>GAHMFKIPGFGKAAANHTPPDMTNMDTRTRHLKVSNCPNNSYALANVAAVSPNDFPNNIYIIIDNLFVFTTRHSNDIPPGTIGFNGNQRTWGGWSLNQDVQAKAFDLFKYSGKQSYLGSIDIDISFRARGKAVSTVFDQDELAKQFVRCYESQIFSPTQYLIMEFQGHFFDLKIRNVQAIDLGDIEPTSAVATGIETKGILTKQTQINFFKGRDGLVNLKSSNSLRPRSNAVIRPDFKFEDLGVGGLDKEFTKIFRRAFASRIFPPSVIEKLGISHVKGLLLYGPPGTGKTLIARKIGTMLNAKEPKIVNGPEILSKYVGSSEENIRNLFKDAEAEYRAKGEESSLHIIIFDELDSVFKQRGSRGDGTGVGDNVVNQLLAKMDGVDQLNNILVIGMTNRKDLIDSALLRPGRFEVQVEIHLPDEKGRLQIFDIQTKKMRENNMMSDDVNLAELAALTKNFSGAEIEGLVKSASSFAINKTVNIGKGATKLNTKDIAKLKVTREDFLNALNDVTPAFGISEEDLKTCVEGGMMLYSERVNSILKNGARYVRQVRESDKSRLVSLLIHGPAGSGKTALAAEIALKSGFPFIRLISPNELSGMSESAKIAYIDNTFRDAYKSPLNILVIDSLETLVDWVPIGPRFSNNILQMLKVALKRKPPQDRRLLIMTTTSAYSVLQQMDILSCFDNEIAVPNMTNLDELNNVMIESNFLDDAGRVKVINELSRSCPNFNVGIKKTLTNIETARHDEDPVNELVELMTQSA[6x];>GMSDPVELLKRAEKKGVPSSGFMKLFSGSDSYKFEEAADLCVQAATIYRLRKELNLAGDSFLKAADYQKKAGNEDEAGNTYVEAYKCFKSGGNSVNAVDSLENAIQIFTHRGQFRRGANFKFELGEILENDLHDYAKAIDCYELAGEWYAQDQSVALSNKCFIKCADLKALDGQYIEASDIYSKLIKSSMGNRLSQWSLKDYFLKKGLCQLAATDAVAAARTLQEGQSEDPNFADSRESNFLKSLIDAVNEGDSEQLSEHCKEFDNFMRLDKWKITILNKIKESIQQQEDDLL[3x];> GASHMSSSTPFDPYALSEHDEERPQNVQSKSRTAELQAEIDDTVGIMRDNINKVAERGERLTSIEDKADNLAVSAQGFKRGANRVRKAMWYKDLKMK;> GASHMSYNNPYQLETPFEESYELDEGSSAIGAEGHDFVGFMNKISQINRDLDKYDHTINQVDSLHKRLLTEVNEEQASHLRHSLDNFVAQATDLQFKLKNEIKSAQRDGIHDTNKQAQAENSRQRFLKLIQDYRIVDSNYKEENKEQAKRQYMIIQPEATEDEVEAAISDVGGQQIFSQALLNANRRGEAKTALAEVQARHQELLKLEKSMAELTQLFNDMEELVIEQQENVDVIDKNVEDAQLDVEQGVGHTDKAVKSARKARKNKIR;> GASHIKFTKQSSVASTRNTLKMAQDAERAGMNTLGMLGHQSEQLNNVEGNLDLMKVQNKVADEKVAELKKLNRSILAVHVSNPFNSKRRRREREEQLKNRKIEEKLMREQTSQQLSQSTQRIEGAMNANNNISEVRERYQRKNVLEKAKRYQFENDEEDDEMELEIDRNLDQIQQVSNRLKKMALTTGKELDSQQKRLNNIEESTDDLDINLHMNTNRLAGI

SNARE (soluble N-ethylmaleimide-sensitive factor (NSF) attachment protein receptor) proteins drive membrane fusion at different cell compartments as their core domains zipper into a parallel four-helix bundle. After fusion, these bundles are disassembled by the AAA+ (ATPase associated with diverse cellular activities) protein Sec18/NSF and its adaptor Sec17/α-SNAP to make them available for subsequent rounds of membrane fusion. The disassembly requires multiple ATP hydrolysis events in the presence of Mg2+; as few as six ATP hydrolysis events are sufficient. The side-loading and side-release mechanism explains how Sec18/NSF can disassemble SNAREs with constrained topologies.

We chose the Sso1–Sec9–Snc1/Snc2 complex (referred to as the ySNARE complex) because each component of this complex crosslinked with high confidence to the D2 domain of Sec18 (Snc1 is highly homologous to Snc2). We prepared the y20S complex in a nonhydrolyzing condition and, after single-particle cryo-EM data collection and processing, we obtained 381,591 high-quality particles that yielded eight three-dimensional (3D) classes into which models were built. In the structures of all eight classes, Sso1 is threaded through the D1 pore of Sec18. A characteristic phenylalanine side-chain density in Sso1 is present at the same position relative to Sec18 in all classes, allowing for reliable indexing of Sso1. The nucleotide states and the arrangements of D1 around the substrate were also the same among all eight classes, with the ADP-engaged E protomer forming the top of a spiral staircase of tyrosine residues. Protomers D, B and C were all ATP bound and formed the middle of the staircase. The bottom protomer, A, formed the base of the staircase. Protomer F, with no apparent density for nucleotide in D1, was not associated with Sso1. Given that this charge distribution is replicated between each pair of D2 subdomains around the D2 surface, it is unsurprising that the Habc domain adopts multiple corresponding rotational states over the eight classes, presumably because of the flexible linker that follows it.>SYYIDADLLREIKQHLKQQQEGLSHLISIIKDDLEDIKLV[2x];> SAPADYFRILVQQFEVQLQQYRQQIEELENHLAT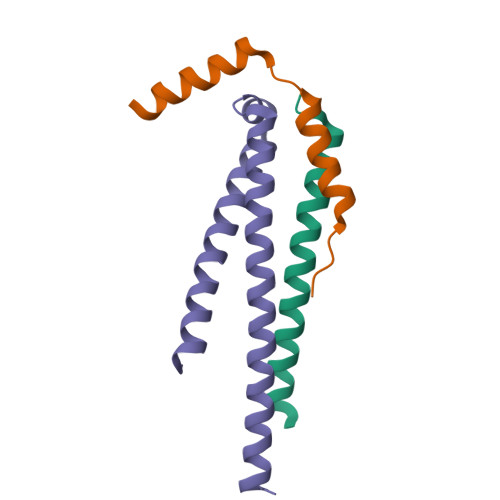QANNSHITPQDLSMAMQKIYQTFVALAAQLQSIHENVKVLKEQYLGYRKMFLG A plant called Arabidopsis thaliana has a light-sensitive protein called ZEITLUPE (or ZTL for short) that helps it keep its circadian clock in sync with the cycle of night and day. In Arabidopsis thaliana, three LOV domain containing proteins ZTL, FLAVIN-BINDING, KELCH REPEAT, F-BOX 1 (FKF1), and LOV KELCH PROTEIN 2 (LKP2) act in circadian timing and seasonal flowering. Recent research indicates that their divergent roles in the circadian clock and photoperiodic flowering may enable interrogation of how chemistry regulates PAS/LOV protein function to select for signaling pathways. These proteins retain analogous elements, where an N-terminal LOV domain regulates activity of a C-terminal E3 ubiquitin ligase to target clock proteins for degradation in a time dependent manner. LOV domains are typified by blue-light induced formation of a C4a adduct between a conserved Cys residue and a bound flavin (FAD, FMN or riboflavin) cofactor.

Towards these aims we solved 2.5 Å, 2.6 Å, and 2.1 Å crystal structures of dark-state WT ZTL, G80R and V48I:G80R (residues 29–165) respectively. Consistent with solution studies, the crystallographic lattice is defined by two sets of anti-parallel dimers formed by extensive contacts along the β-scaffold. We term these interfaces the ‘compact’ and ‘elongated’ dimers based on a 2 Å translation that is coupled to the degree of order present within the Ncap. In contrast to other LOV proteins, where a conserved Gln (Q154) acts as a molecular bridge linking the FMN to a residue in Aβ, the dark-state structure of ZTL contains a heterogeneous orientation of the active site Q154. The altered orientation is coupled to contacts in the Ncap, Ccap and helical interface. In ZTL, Q154 does not adopt a specific orientation as observed in all other LOV structures, rather it varies in all four molecules in the asymmetric unit of both WT-ZTL and G80R. The lack of a side chain at G46 permits favorable interactions for Q154 at the flavin O4 position and allows insertion of F156 into the flavin active site. In this manner an unusual orientation of Q154 links the Iβ-Ccap hinge and helical interface through a QFF motif (Q154-F155-F156). In our ZTL structures this is not the case, rather dark-state structures have a heterogeneous orientation of Q154 that samples orientation near both the buried conformation and an exposed conformation. Rather, we propose that steric interactions involving the flavin O4 position and G46 shift a dynamic equilibrium in the Q154 position to stabilize the ZTL protein in a light-state configuration.

>[4x]GGPIPYPVGNLLHTAPCGFVVTDAVEPDQPIIYVNTVFEMVTGYRAEEVLGGNCRFLQCRGPFAKRRHPLVDSMVVSEIRKCIDEGIEFQGELLNFRKDGSPLMNRLRLTPIYGDDDTITHIIGIQFFIETDIDLGP>GAPATVTEQGE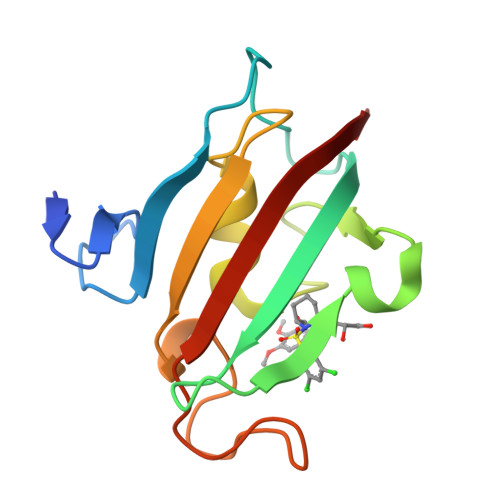DITSKKDRGVLKIVKRVGNGEETPMIGDKVYVHYKGKLSNGKKFDSSHDRNEPFVFSLGKGQVIKAWDIGVATMKKGEICHLLCKPEYAYGSAGSLPKIPSNATLFFEIELLDFKGE[2x]> MAHHHHHHAREPISLDQTIGDEGDSQLGDF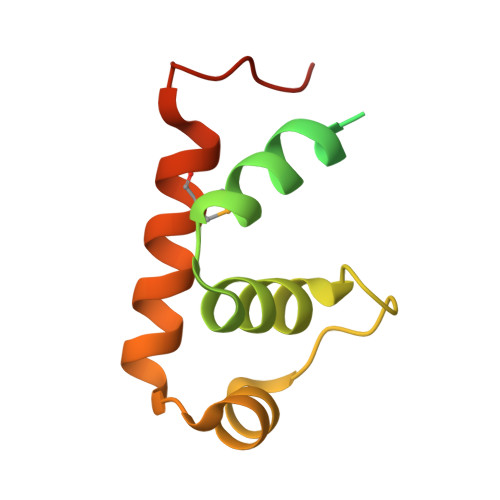IEDSEAVVAVDAVSFTLLQDQLQSVLDTLSEREAGVVRLRFGLTDGQPRTLDEIGQVYGVTRERIRQIESKTMSKLRHPSRSQVLRDYLD The T4BS secretion coupling complex of L. pneumophila comprises the inner membrane AAA+ ATPase DotL (IcmO) and two inner membrane/cytoplasmic components, DotM (IcmP) and DotN (IcmJ). In this study, we determine the crystal structure of the cytoplasmic domain of DotM and observe large patches of basic residues, leading us to hypothesize that DotM might form the recruiting platform for Glu-rich motif-containing effectors. Our results suggest that DotM’s cytoplasmic domain is capable of binding directly another subgroup of Legionella effectors that contain acidic Glu-rich motifs at their C terminus.

Further binding studies were conducted with several DotM mutants, where Arg residues (single or double) on the protein’s surface were mutated to Glu. Five mutants were produced: R196E/R197E (termed “M1”), R314E/R315E (termed “M2”), R347E/R348E (termed “M3”), R217E (termed “M4”), and R262E (termed “M5”). Binding was abrogated in M1, M2, and M4, indicating that these Arg patches are involved in binding of acidic Glu-rich peptides. M3 and M5 were unaffected suggesting that they are not involved in Glu-rich sequence binding. The Lpg1663 and the consensus OSM peptide was also assessed for binding to the M1 and M2 mutants and binding was found to be also abrogated (Fig. 4 and Table 3; Lpg1663- or OSM-binding to other mutants was not tested because wild-type DotM, M1 and M2 display the same binding behavior for the Lpg1663 and OSM peptides as for CegC3). To ascertain that the observed binding deficiency in M1, M2, and M4 variant proteins was not due to folding defects caused by the mutations, these three proteins were crystallized and their structures were determined and shown to be virtually identical to the wild-type protein. Thus, the mutations do not introduce structural defects, suggesting that the ITC binding results reflect an effective role of the residues in binding. Other interactions are between residues R196 and R197 of DotM and CegC3 E145 and a stacking interaction between these two residues and the side chain of CegC3 F146. Remarkably (given that acidic Glu-rich motif-containing effectors represent only a subset of Legionella effectors), the M1 and M4 mutations resulted in a significant decrease in L. pneumophila replication in the macrophages (up to 70–80%). However, in A. castellanii, M1 reduces intracellular growth by up to 90% (after 24 h) while the slight reduction in intracellular growth of the M4 mutant is not statistically significant. We observed that the M1 and M4 dotM mutants producing the reporter fusions Cya-CegC3Cter, Cya-OSSCter, or Cya-Lpg1663Cter displayed lower levels of effector translocation compared to the wild-type strain of L. pneumophila (Cya-CegC3Cter: 50% and 30% decrease compared to wild-type DotM for M1 and M4, respectively; Cya-OSSCter: 50% and 40% decrease compared to wild-type DotM for M1 and M4, respectively; Cya-Lpg1663Cter: 60% and 55% decrease compared to wild-type DotM for M1 and M4, respectively).

>[2x]GPSGGGADVNKGPWAMALTPMEFARKYNLLRKDDALLDNPVPGEEMTAGIEEGDAKRVFTMQLGPYWDGFERCSPQAYALSAVFMARMNRDRDAANNILKVLDKTFVDGKPDFSVARPVMKKYQNSELVQEVVAKHAYVLTVIASLLEAAREDGVVPSSEFLWLKPVDRRLWYMLNCVGRQTPYSEVAGPFAHWKAEKEMGRRSLVPMIDEAIRALEIAVKEVRLTPRQMEELEP>AHHHHHHGSIRASKRALSVEYAIRDVVLPARELEKKGIKVIRLNIGDPVKFDFQPPEHMKEAYCKAIKEGHNYYGDSEGLPELRKAIVEREKRKNGVDITPDDVRVTAAVTEALQLIFGALLDPGDEILVPGPSYPPYTGLVKFYGGKPVEYRTIEEEDWQPDIDDIRKKITDRTKAIAVINPNNPTGALYDKKTLEEILNIAGEYEIPVISDEIYDLMTYEGEHISPGSLTKDVPVIVMNGLSKVYFAT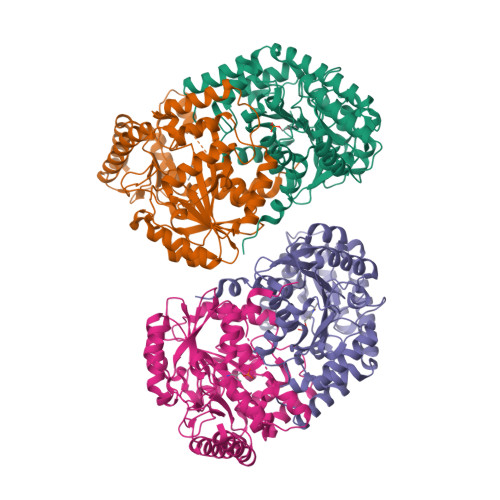GWRLGYMYFVDPENKLSEVREAIDRLARIRLCPNTPAQFAAIAGLTGPMDYLKEYMKKLKERRDYIYKRLNEIPGISTTKPQGAFYIFPKIEVGPWKNDKEFVLDVLHNAHVLFVHGSGFGEYGAGHFRAVFLPPIEILEEAMDRFEKFMKERLKE[4x]> MIIIRYLVRETLKSQLAILFILLLIFF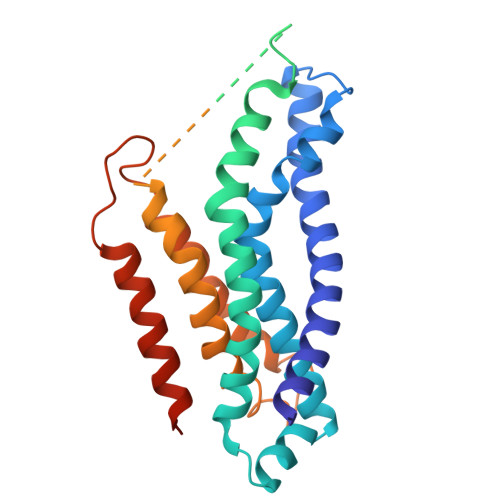CQKLVRILGAAVDGDIPTNLVLSLLGLGIPEMAQLILPLSLFLGLLMTLGKLYTESEITVMHACGLSKAVLIKAAMILALFTGAVAAVNVMWAGPWSSRHQDEVLAEAKANPGMAALAQGQFQQASDGNAVMFIESVNGNRFHDVFLAQLRPKGNARPSVVVADSGELSQQKDGSQVVTLNKGTRFEGTAMLRDFRITDFNNYQAIIGHQAVSADPDDTEQMDMRTLWKTHTDRARAELHWRFTLVATVFIMALMVVPLSVVNPRQGRVLSMLPAMLLYLVFFLLQTSIKSNGGKGKMDPAIWMWAINLLYFALAVLLNLWDTVPMRRFRARFNKGAA> GSMTTTETPKTISLTWVGTFVDQRVREIQEGYRLDNPRAVATLARLRRGAGKEIGDTPDLWGLILDDRFYADAPPLKEKDMEVAENSAHIALTLYAIHQQSRRDDRMHQRGWGL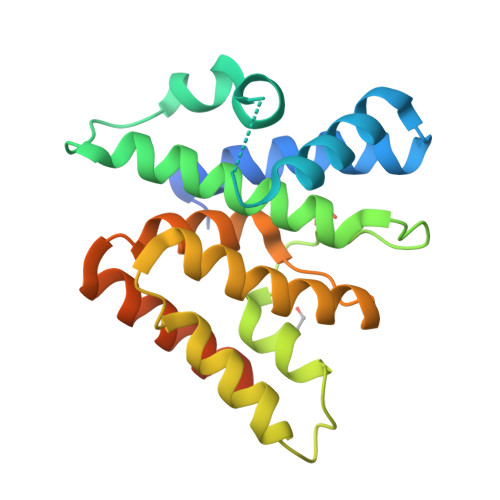GEAVRRLMPSSEIDEPLRKRFVQVGHAVTYKALAQRLREIVTLLRRDAIPLDYGLLADQLYQFRTPQGAQRVRTAWGRGFHAYRPKTTQNPDSTTTTEKDNS> MVPISPIETVPVKLKPGMDGPKVKQWPLTEEKIKALVEICTEMEKEGKISKIGPENPYNTPVFAIKKKDSTKWRKLVDFRELNKRTQDFWEVQLGIPHPAGLKKKK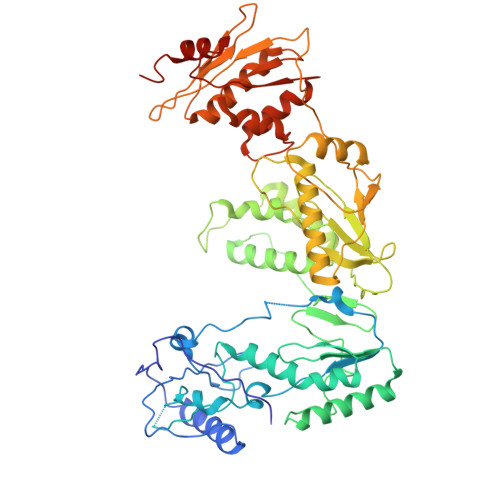SVTVLDVGDAYFSVPLDEDFRKYTAFTIPSINNETPGIRYQYNVLPQGWKGSPAIFQSSMTKILEPFKKQNPDIVIYQYMDDLYVGSDLEIGQHRTKIEELRQHLLRWGLTTPDKKHQKEPPFLWMGYELHPDKWTVQPIVLPEKDSWTVNDICKLVGKLNWASQIYPGIKVRQLSKLLRGTKALTEVIPLTEEAELELAENREILKEPVHGVYYDPSKDLIAEIQKQGQGQWTYQIYQEPFKNLKTGKYARMRGAHTNDVKQLTEAVQKITTESIVIWGKTPKFKLPIQKETWETWWTEYWQATWIPEWEFVNTPPLVKLWYQLEKEPIVGAETFYVDGAANRETKLGKAGYVTNKGRQKVVPLTNTTNQKTQLQAIYLALQDSGLEVNIVTDSQYALGIIQAQPDKSESELVNQIIEQLIKKEKVYLAWVPAHKGIGGNEQVDKLVSAGIRKILDLGTLVPR(11Z,13Z)-hexadeca-11,13-dien-1-ol | C16 H30 O | 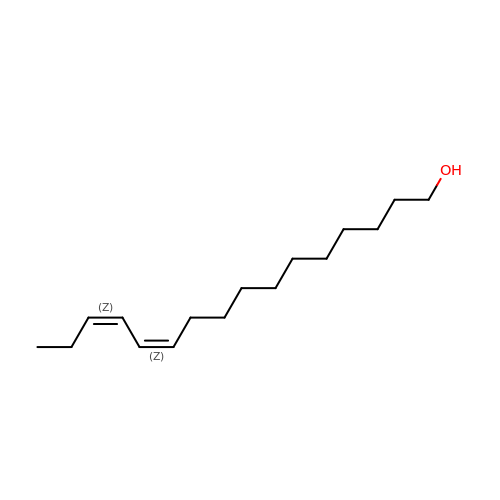GKFQVSXEEVMHMA-OUPQRBNQSA-N4-[2-[(phenylmethyl)amino]ethyl]benzene-1,2-diol | C15 H17 N O2 | 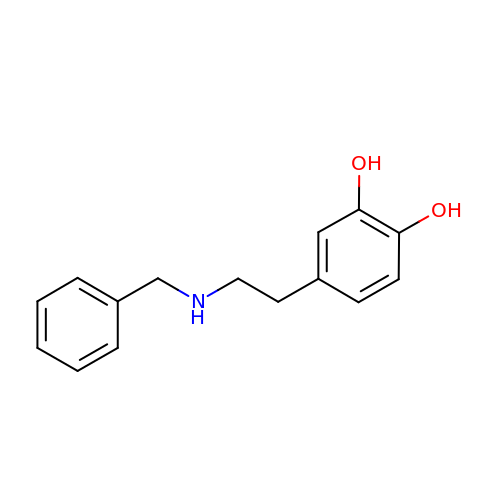VFXBAOSXGMLCEF-UHFFFAOYSA-N3-fluoro-6-(4-fluorophenyl)-2-hydroxy-6-oxohexa-2,4-dienoic acid | C12 H8 F2 O4 | 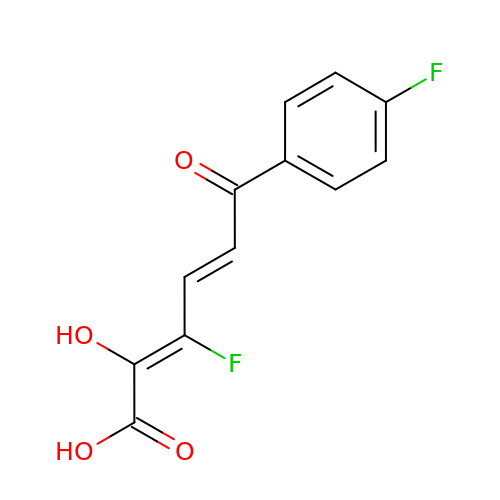CPZFGNOKCMJZFO-BTHQEHEQSA-N>HMSDVSLKLSAKDIYEKDFEKTMARGYRREEVDAFLDDIIADYQKMADMNNEVVKLSEENHKLKKELEELR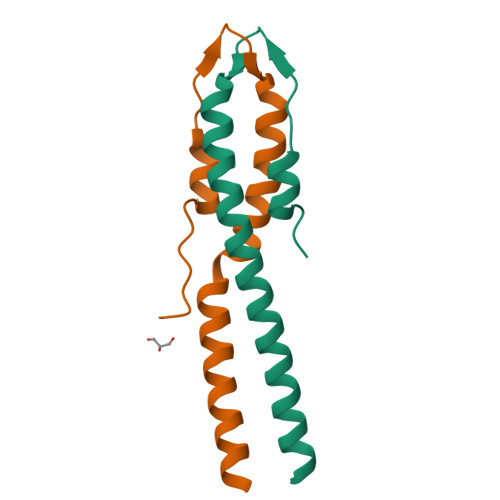[4x]> GPGSEFLDGDLDPGLPSTEDVI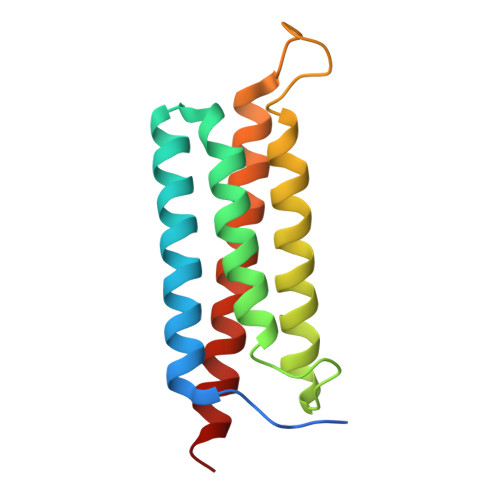LKTEQVTKNIQELLRAAQEFKHDSFVPCSEKIHLAVTEMASLFPKRPALEPVRSSLRLLNASAYRLQSECRKTVPPEPGAPVDFQLLTQQVIQCAYDIAKAAKQLVTITTREKKQ> MAEYQDKVVDVEVSLGTQPIDTVGFETPMFLAMHGNFPERIRFYVSTAGMVADGFAVGSPAYQFATNAFAGNFAPQRV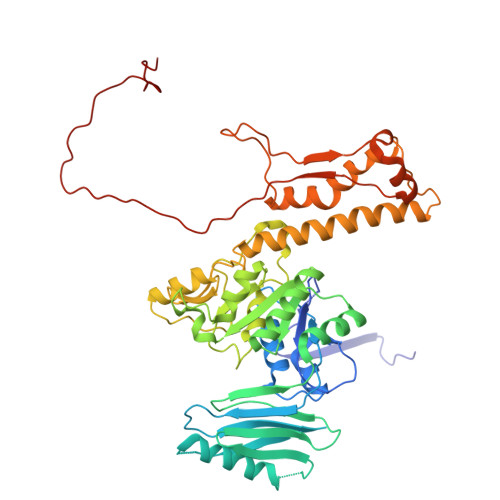AIGRMSIDSSKVDFTGTTNTEQVVVNITLNKVVKAVKINVLPGNTPAQIATALADAVTADADLTGKATAVATGTYVTVTAVSPNVVSVGKGAGVYKIVNESSETVATVLPSVIAENHNWYFLATEARSDADIVAAAEFAKANYKLHIYNSTDVDAYAPENSAASVFDTLKSLSYDSLGTSDAGADVDFTEGSVIGAMAANDPSYGDSLHLKTMPGMVPFAGSDTQRSNAWSRNANIYRGLYGGGSYIEGKTSSGQYVDVIRFSHWVKFRMEESVFAYMKRRSDMGLSMKMSDEDLPVLKSVLMNNPINIGIRNGGILTGYDTENKVSYDPTIIIPKRANIPTNDLAARILRDVKVELVYNNSLHYVKIRASVVLDRPAGQSTNAQTPMSSSAVGV>[4x]SASASAMLSRKGIIPEEYVLTRLAEDPAEPRYRARQRRARFVSKKGNCNVAHKNIREQGRFLQDVFTTLVDLKWPHTLLIFTMSFLCSWLLFAMAWWLIAFAHGDLAPSEGTAEPCVTSIHSFSSAFLFSIEVQVTIGFGGRMVTEECPLAILILIVQNIVGLMINAIMLGCIFMKTAQAHRRAETLIFSKHAVIALRHGRLCFMLRVGDLRKSMIISATIHMQVVRKTTSPEGEVVPLHQVDIPMENGVGGNSIFLVAPLIIYHVIDANSPLYDLAPSDLHHHQDLEIIVILEGVVETTGITTQARTSYLADEILWGQRFVPIVAEEDGRYSVDYSKFGNTIKVPTPLCTARQLDEDHSLLEALTLASARGPLRKRSVPMAKAKPKFSISPDSLSSNSLEVLFQG;>MPLAFCGSENHSAAYRVDQGVLNNGCFVDALNVVPH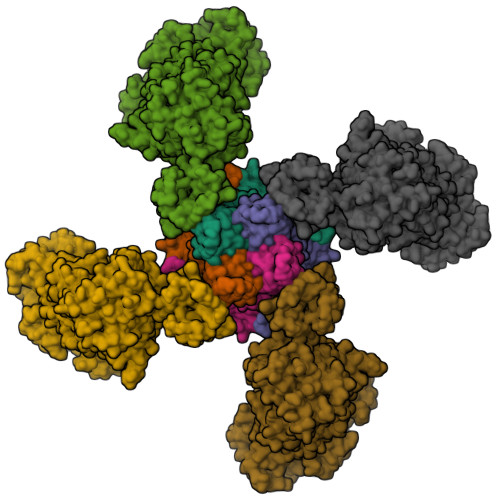VFLLFITFPILFIGWGSQSSKVHIHHSTWLHFPGHNLRWILTFMLLFVLVCEIAEGILSDGVTESHHLHLYMPAGMAFMAAVTSVVYYHNIETSNFPKLLIALLVYWTLAFITKTIKFVKFLDHAIGFSQLRFCLTGLLVILYGMLLLVEVNVIRVRRYIFFKTPREVKPPEDLQDLGVRFLQPFVNLLSKGTYWWMNAFIKTAHKKPIDLRAIGKLPIAMRALTNYQRLCEAFDAQVRKDIQGTQGARAIWQALSHAFGRRLVLSSTFRILADLLGFAGPLCIFGIVDHLGKENDVFQPKTQFLGVYFVSSQEFLANAYVLAVLLFLALLLQRTFLQASYYVAIETGINLRGAIQTKIYNKIMHLSTSNLSMGEMTAGQICNLVAIDTNQLMWFFFLCPNLWAMPVQIIVGVILLYYILGVSALIGAAVIILLAPVQYFVATKLSQAQRSTLEYSNERLKQTNEMLRGIKLLKLYAWENIFRTRVETTRRKEMTSLRAFAIYTSISIFMNTAIPIAAVLITFVGHVSFFKEADFSPSVAFASLSLFHILVTPLFLLSSVVRSTVKALVSVQKLSEFLSSAEIREEQCAPHEPTPQGPASKYQAVPLRVVNRKRPAREDCRGLTGPLQSLVPSADGDADNCCVQIMGGYFTWTPDGIPTLSNITIRIPRGQLTMIVGQVGCGKSSLLLAALGEMQKVSGAVFWSSLPDSEIGEDPSPERETATDLDIRKRGPVAYASQKPWLLNATVEENIIFESPFNKQRYKMVIEACSLQPDIDILPHGDQTQIGERGINLSGGQRQRISVARALYQHANVVFLDDPFSALDIHLSDHLMQAGILELLRDDKRTVVLVTHKLQYLPHADWIIAMKDGTIQREGTLKDFQRSECQLFEHWKTLMNRQDQELEKETVTERKATEPPQGLSRAMSSRDGLLQDEEEEEEEAAESEEDDNLSSMLHQRAEIPWRACAKYLSSAGILLLSLLVFSQLLKHMVLVAIDYWLAKWTDSALTLTPAARNCSLSQECTLDQTVYAMVFTVLCSLGIVLCLVTSVTVEWTGLKVAKRLHRSLLNRIILAPMRFFETTPLGSILNRFSSDCNTIDQHIPSTLECLSRSTLLCVSALAVISYVTPVFLVALLPLAIVCYFIQKYFRVASRDLQQLDDTTQLPLLSHFAETVEGLTTIRAFRYEARFQQKLLEYTDSNNIASLFLTAANRWLEVRMEYIGACVVLIAAVTSISNSLHRELSAGLVGLGLTYALMVSNYLNWMVRNLADMELQLGAVKRIHGLLKTEAESYEGLLAPSLIPKNWPDQGKIQIQNLSVRYDSSLKPVLKHVNALIAPGQKIGICGRTGSGKSSFSLAFFRMVDTFEGHIIIDGIDIAKLPLHTLRSRLSIILQDPVLFSGTIRFNLDPERKCSDSTLWEALEIAQLKLVVKALPGGLDAIITEGGENFSQGQRQLFCLARAFVRKTSIFIMDEATASIDMATENILQKVVMTAFADRTVVTIAHRVHTILSADLVIVLKRGAILEFDKPEKLLSRKDSVFASFVRADK[4x]> SHGMAVTKVTVDGIEFPPTITPPGSSKSLTLLGAGVRGIEIEAIQIKVTAIGVYAEPEVIASHLQ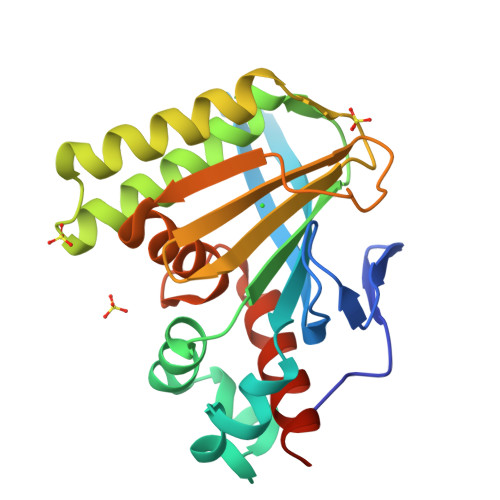KWKGKSASELVEDDGFFKDLVQAPVEKLVKITMIKGLTGSQYGGAVEENIKDRLAALDKYSEAEEEALEEFREFFKTKSFPKGSVIFFHWSSPSTLQISVSTDGSLPEEAEATVENANVAAALLDVFLGKNSVSPSTKASVAEGISALLMKNKDEKEV> GPGHMTTLTRQDLNFGQVVADVLCEFLEVAVHLILYVREVYPVGIFQKRKKYNVPVQMSCHPELNQYIQDTLHCVKPLLEKNDVEKVVVVILDKEHRPVEKFVFEITQPPLLSISSDSLLSHVEQLLAAFILKISVCDAVLDHNPPGCTFTVLVHTREAATRNMEKIQVIKDFPWILADEQDVHMHD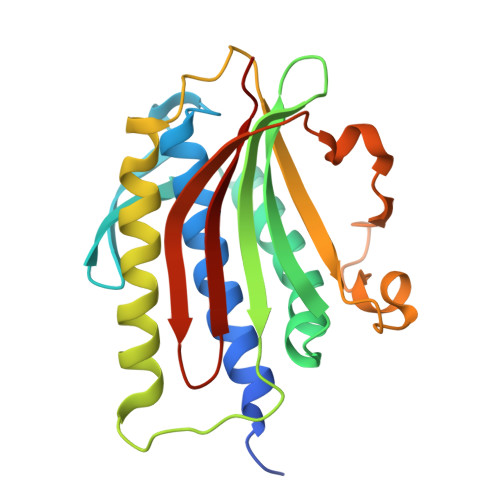PRLIPLKTMTSDILKMQLYVEERAHKGS The export apparatus consists of an export gate complex formed by 5 highly conserved transmembrane proteins (FlhA, FlhB, FliP, FliQ, and FliR) and a cytoplasmic ATPase complex consisting of FliH, FliI, and FliJ [1–4]. FliP is a 25-kDa transmembrane protein that has a cleavable N-terminal signal peptide, 4 transmembrane (TM) helices, and a relatively large periplasmic domain (FliPP) between TM-2 and TM-3. Here we report that FliP forms a homohexameric ring with a diameter of 10 nm. In summary, we have presented direct evidence that FliP forms a homohexamer with the help of the FliO complex and that FliPP–FliPP and FliPP–FliO interactions are required for efficient FliP6 ring formation.

Although no St-FliPP crystal was obtained, the Tm-FliPP crystals were grown, and its structure was solved at 2.4 Å resolution. There are 2 tetramers in the asymmetric unit, and their structures are essentially identical. The 8 Tm-FliPP molecules in the asymmetric unit show no significant structural difference (root mean square distances for Cα atoms are less than 0.46 Å for the 8 molecules). Tm-FliPP monomer consists of 3 α-helices: α1, α2 and α3. The N-terminal 13 residues are invisible in the electron density map presumably because of their conformational flexibility. Therefore, the atomic model of Tm-FliPP contains residues from Thr-122 to Lys-188. Since each subunit of the Tm-FliPP tetramer is related by D2 symmetry, we studied 3 possible intermolecular interactions: between Mol A and Mol B (Mol C and Mol D), between Mol A and Mol C (Mol B and Mol D), and between Mol A and Mol D (Mol B and Mol C). The A–B interaction is hydrophobic, and Tyr-124, Phe-128, Met-154, Leu-155, Pro-176, and Leu-180 are involved in this interaction (S7A, S7C). The A–C interaction contains both hydrophilic and hydrophobic nature, and Met-127, Arg-130, Val-131, Arg-134, Phe-138, Glu-142, Glu-182, Val-185, Ala-186, and Phe-187 are responsible (S7B, S7F). There is no direct contact between Mol A and Mol D. Since sedimentation equilibrium analytical ultracentrifugation measurements have revealed that Tm-FliPP forms a homotetramer in solution, we conclude that the tetramer structure observed in the crystal appears to be equivalent to that in solution.

>GSHYNNAITPYLNKETGYQEMFQRVNTRIREFMINELKNHHNEDNVFMLAKNSGIEIAKIEEAPNAVLIPAFVLGELEVAFK[8x]> MNDSSVIYRAIVTSKFRTEKMLNFYNSIGSGPDKNTIFITFGRSEPWSSNENEVGFAPPYPT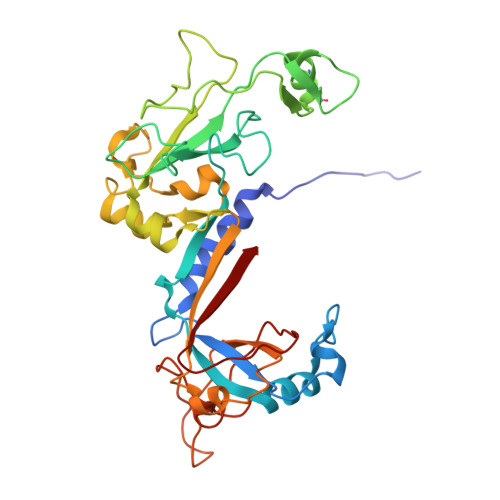DSVLGVTDMWTHMMGTVKVLPSMLDAVIPRRDWGDTRYPDPYTFRINDIVVCNSAPYNATESGAGWLVYRCLDVPDTGMCSIASLTDKDECLKLGGKWTPSARSMTPPEGRGDAEGTIEPGDGYVWEYLFEIPPDVSINRCTNEYIVVPWPEELKEDPTRWGYEDNLTWQQDDFGLIYRVKANTIRFKAYLDSVYFPEAALPGNKGFRQISIITNPLEAKAHPNDPNVKAEKDYYDPEDLMRHSGEMIYMENRPPIIMAMDQTEEINILFTF>MESKALLLLALSVCLQSLTVSRGGLVAADRITGGKDFRDIESKFALRTPEDTAEDTCHLIPGVTESVANCHFNHSSKTFVVIHGWTVTGMYESWVPKLVAALYKREPDSNVIVVDWLSRAQQHYPVSAGYTKLVGQDVAKFMNWMADEFNYPLGNVHLLGYSLGAHAAGIAGSLTNKKVNRITGLDPAGPNFEYAEAPSRLSPDDADFVDVLHTFTRGSPGRSIGIQKPVGHVDIYPNGGTFQPGCNIGEALRVIAERGLGDVDQLVKCSHERSVHLFIDSLLNEENPSKAYRCNSKEAFEKGLCLSCRKNRCNNMGYEINKVRAKRSSKMYLKTRSQMPYKVFHYQVKIHFSGTESNTYTNQAFEISLYGTVAESENIPFTLPEVSTNKTYSFLLYTEVDIGELLMLKLKWISDSYFSWSNWWSSPGFDIGKIRVKAGETQKKVIFCSREKMSYLQKGKSPVIFVKCHDKSLNRKSG[2x]

Lipoprotein lipase (LPL) is a secreted enzyme that is active in the capillaries, where it hydrolyzes triglycerides found in chylomicrons and very low-density lipoproteins (VLDL) to release FFA, which are transported across the capillary endothelial membrane as a source of energy. In addition to acting on triglycerides, LPL has phospholipase activity, making it essential to regulate where and when LPL is active to prevent off-target hydrolysis events. Active LPL is needed to prevent hypertriglyceridemia, which is a risk factor for cardiovascular disease (CVD). Independent from its role hydrolyzing triglycerides, LPL on TRLs mediates lipoprotein remnant uptake by the liver.

Using cryogenic electron microscopy (cryoEM), we determined the structure of an active LPL dimer at 3.9 Å resolution. The structure shows that LPL forms a homodimer associated at the C-terminal domains (“tails”) of both subunits. The active LPL dimer is oriented with both its substrate recognizing tryptophan loops and active sites facing the same direction, suggesting an active conformation that could be engaged with a TRL substrate. Analysis of the homodimerization interface shows significant overlap with the LPL/GPIHBP1 interface and the LPL helical interfaces. This suggests that LPL homodimerization, binding to GPIHBP1, and LPL helix formation are all mutually exclusive states. Indeed, we see that the density corresponding to the lid residues in our map are shifted away from the opening of the active site. We thus analyzed the LPL active site in the structure and found a clearly defined pore traversing LPL which is directly adjacent to the active site residues. The pore in the dimer structure has a bottleneck with a radius of 1.4 Å, which is sufficient for the carbon hydrogen backbone of a fatty acid. The pore has a highly hydrophobic section that could accommodate a fatty acid tail, potentially aligning the hydrolysable ester bond with the active site residues in a relatively more hydrophilic section of the pore entrance.>MKETILVNLVSEQTIPNVQFIKWYFNKKQTPMKILLVSTKEMEQKEKSLFIKNALHFSDSFVEWETIHTDGNDISKTENILTDYFRDNEYKNIIVNITGGTKIMSLAAFDFFNNKPNTEIFYQPIGKELQELYPNKQKYDMF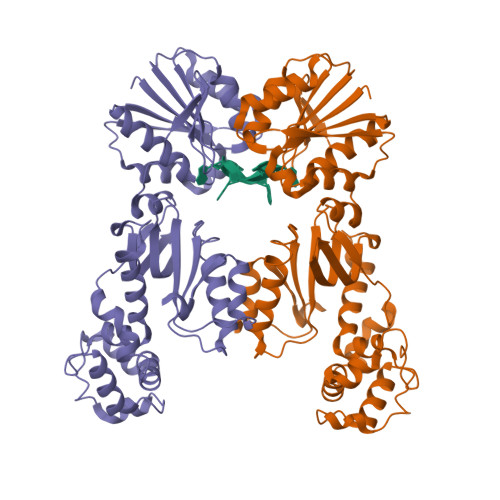EVLSLKEYLDAHGISYKYDNECVKDWNYNKTVYDLCVADNRELIKGMIALQNNSYFNNVYKRKDFLDFTQIEEEKFIAINHPAATKENMIKILQIFGFDVSRIEHKHIRYITGGWFEEYVYQKICNEYHNVDEKNVALNVTIQKGNDKNELDVIYLDKDNKLHVIECKSFVDGNEGNRVLNDALYKLQAIIKSKFGLYVKQHLYTKSIIEKETPLNRAKEFGIDIKDGTQLGSGHHHHHH[2x]>REDYSLECDPAVIGTAVKGKEAVHSDLGYWIESEKNDTWRLKRAHLIEMKTCEWPKSHTLWTDGIEESDLIIPKSLAGPLSHHNTREGYRTQMKGPWHSEELEIRFEECPGTKVHVEETCGTRGPSLRSTTASGRVIEEWCCRECTMPPL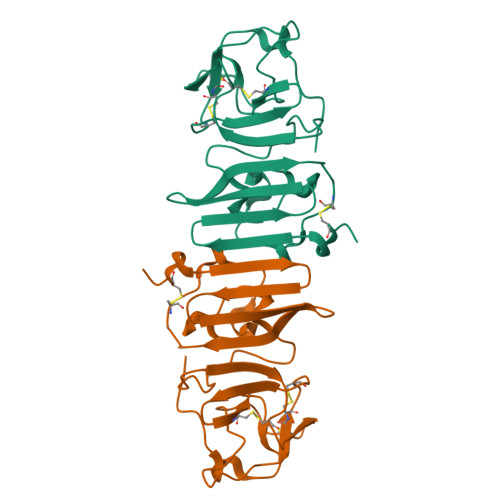SFRAKDGCWYGMEIRPRKEPESNLVRSMVTA[2x]>MKILVIQGPNLNMLGHRDPRLYGMVTLDQIHEIMQTFVKQGNLDVELEFFQTNFEGEIIDKIQESVGSDYEGIIINPGAFSHTSIAIADAIMLAGKPVIEVHLTNIQAREEFRKNSYTGAACGGVIMGFGPLGYNMALMAMVNILAEMKAFQE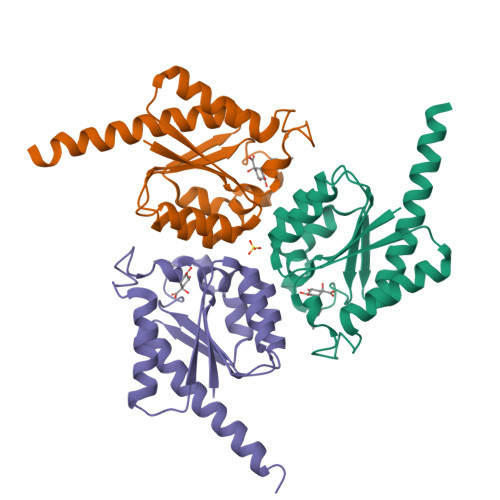AQKNNPNNPINNQK[3x]>[8x]MSEFILTSDKLVWTYDGHKLQIEPWGENSLRVRATVAPELNGNDWALLPAKPSTKVKVSEFEDSARIVNGNISAVVNGRGQLSFYNQNGKLLLEEYWRTRFVAGQGEDTSSKYFSPLTHEARELKPIQGGKFELRARFESQPDERIYGLGQYQQPFLNVKGCTMELAQRNSQASVPFMMSSLGYGMLWNNPAIGEVSFANNVTTWMARVTEQLDYWITAADTPAEISQQYAAATGAAPMLPDYAAGFWQCKLRYRTQDELMEVAREYKRRSLPISVIVADFFHWPNQGDWCFDTREWPDPKAMI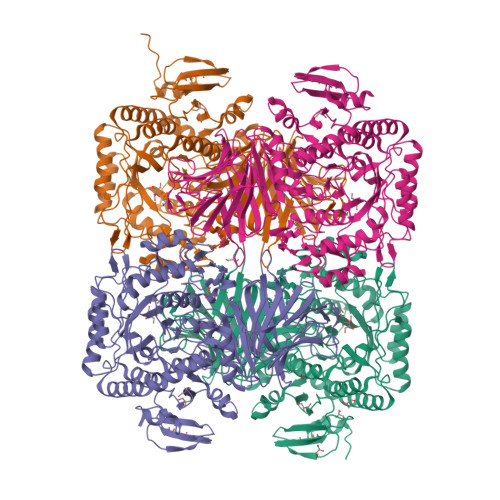DELKEMGIELMVSIWPTVDNRTENYKIMKEKGYLVKAERGVPVTMTFLGNTTFFDATHPGARKYVWEQAKKNYHDLGIKIFWLDEAEPEYSVYDFENYRYHLGPVLEVGNIYPRGYAQAFYEGMEEAGQTEIVNLLRCAWAGSQRYGALVWSGDINSTFGALRNQLMAGLNMGIAGIPWWTTDIGGFDGGDINDPAFQELLIRWFQWGVFCPVTRLHGFRQPMEEPAETYRDGIAQCMTGAANEIWSYGEDNYAIMKSCLELRERLRPYVMRVMKAAHDTGAPVMRPLFFDFPDQAEAWQIEDQYMFGPDILVAPVLEAGQRSRKVWLPEGCAWIDLNTGARQNGGQWCDCDAPLEAIPVFIREAAAVQAELSIALEHHHHHH> MGSSHHHHHHSSGENLYFQGHHMGKKLSLIDFNEIYNEENLITRANPIENHEFSDDGIYSERIFGSYNEDDDDKDIDTIGWINIEPYYIINPILFTIIKKCIPSINKIINYQQSIDQNGENIDLTEEIGEDDYIGLVKFKDNFDDLLEKYTDKKKYQKEYDFLIENHDKIFINKLPVFSHKLRPATLLTGSKGKVLAFDEINNYYNFVIEYINQINEGVV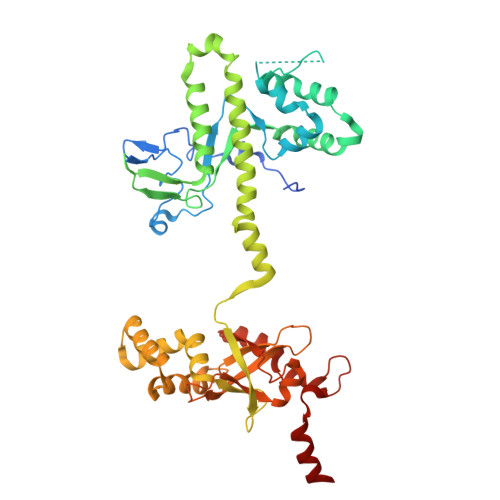SDDSIDLLLLPLLYNMQFYANNILTRIISEYLRGKKGFLRKNIMGSRINFSARNVITPLIGHPIDEVAMPYKTFAELYKFQLINLISKVKGINYNEALKFWEKGILGFNQELYNYMEELITKTKGGCTFLLNRNPTISIGSILYLKIGLIKKDYKDLTLGISNNLLSALSGDYDGDVLNIIPVFDNKMKEHFSLLSPQNFLVDRNNGRFNGDFDLQKDQILGIFILNN>GMMDTVKNRRTIRKYQQKDITPDLLNDLLETSFRASTMGGMQLYSVVVTRDAEKKEILSPAHFNQPMVKEAPVVLTFCADFRRFCKYCQERNAVPGYGNLMSFLNAAMDTLLVAQTFCTLAEEAGLGICYLGTTTYNPQMIIDALHLPELVFPITTVTVGYPAESPKQVDR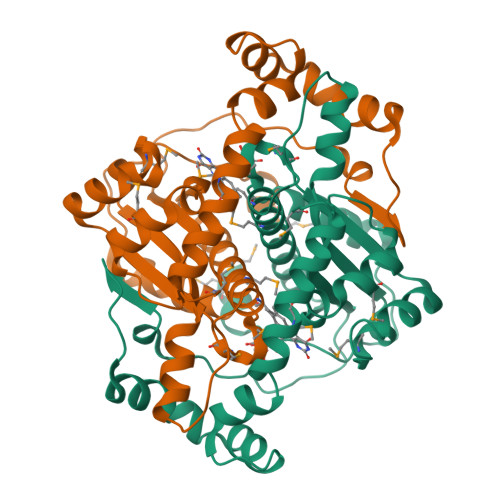LPIEGIIHEESYHDYTAEDINRLYAYKESLPENKLFIEENQKETLPQVFTDVRYTKKDNEFMSENLLKVLRRQGFMD[2x]> MAANPQKIILWYRNDLRLHDHEPLDLATSTQGQIIPLYCFDPRQFAKTSFGFPKTGGFRGKFLLESVADLRHNFQKIGSNLLVRIGEPERVIFDLVKQLNIDAVYYHKEVTAEELAVETALEKALTPLGVEVKSFWGATLYHLKELPFPIEKLPELFTNFRKQVEQKSVIYPPYTPPNQLPQFPDIEPGEIPTLTELGITPAPFDERSVLDFAGGETAGLSRLNDYFWRRDCLKNYKQTRNGMLGSDYSSKFSPWLANGCLSPRWIYQQVQDYQHQRVKNDSTYWLVFELLWRDYFRFICLKHGPKVFYKSGLQGVKIPWGENWEQWQIWCQGLTGFPLVDANMRELAATGFMSNRGRQNVASFLT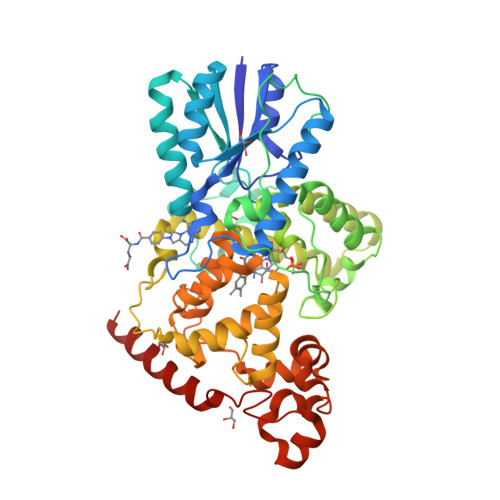KNLGINWQMGAEWFESVLIDYDVCSNWGNWNYTAGVGNDGRGFRYFNIAKQSQDYDPMGDYVKHWLPELASIPDGRVHSPWRLSNQEQIRFGVRLGVDYPYPMVDLQESVEANRRIYEKALRMT2-(1-adamantyl)-~{N}-[7-[1-(phenylmethyl)-5-[(2,4,6-trimethylphenyl)sulfonylamino]benzimidazol-2-yl]heptyl]ethanamide 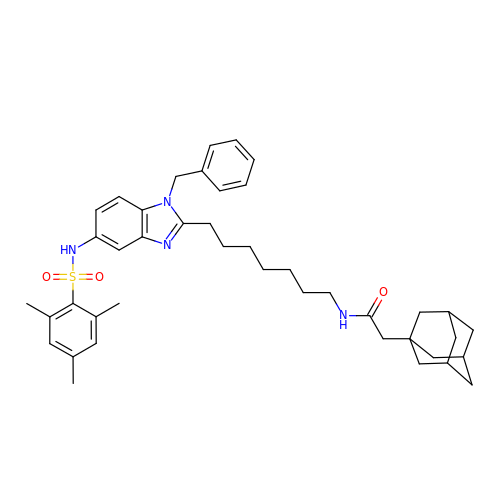| C42 H54 N4 O3 S | ICJUXBWVXRFIBW-UGDOBHGRSA-N N-cyclopropyl-N-(trans-4-pyridin-3-ylcyclohexyl)-4-[(1S)-2,2,2-trifluoro-1-hydroxy-1-methylethyl]benzamide 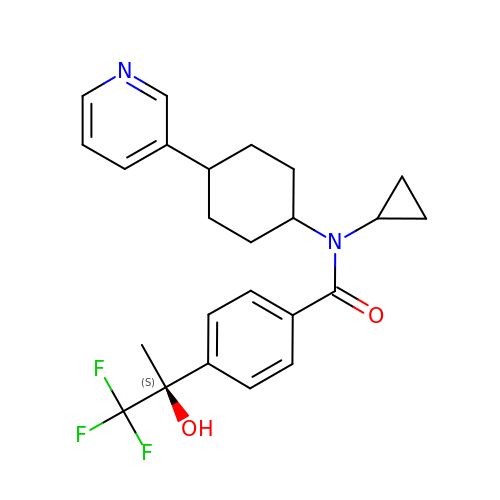| C24 H27 F3 N2 O2 | FLRYWTWLHWACRP-GRWTVWFQSA-N> MGDSILSQAEIDALLNGDSDTKDEPTPGIASDSDIRPYDPNTQRRVVRERLQALEIINERFARQFRMGLFNLLRRSPDITVGAIRIQPYHEFARNLPVPTNLNLIHLKPLRGTGLVVFSPSLVFIAVDNLFGGDGRFPTKVEGREFTHTEQRVINRMLKLALEGYSDAWKAINPLEVEYVRSEMQVKFTNITTSPNDIVVNTPFHVEIGNLTGEFNICLPFSMIEPLRELLVNPPLENSRHEDQNWRDNLVRQVQH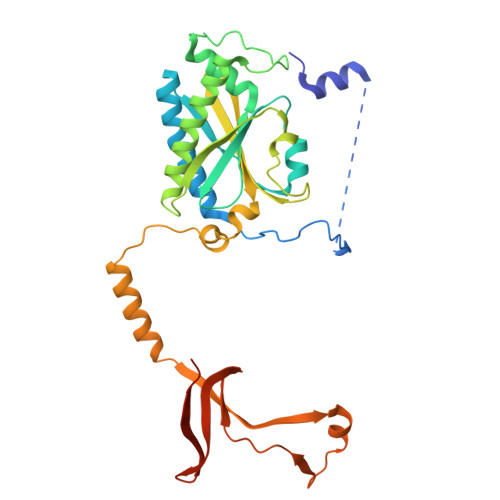SELELVANFADIPLRLSQILKLKPGDVLPIEKPDRIIAHVDGVPVLTSQYGTVNGQYALRVEHLINPILNSLNEEQPK>GSMELLQGKTFVVMGVANQRSIAWGIARSLHNAGAKLIFTYAGERLERNVRELADTLEGQESLVLPCDVTNDEELTACFETIKQEVGTIHGVAHCIAFANRDDLKGEFVDTSRDGFLLAQNISAFSLTAVAREAKKVMTEGGNILT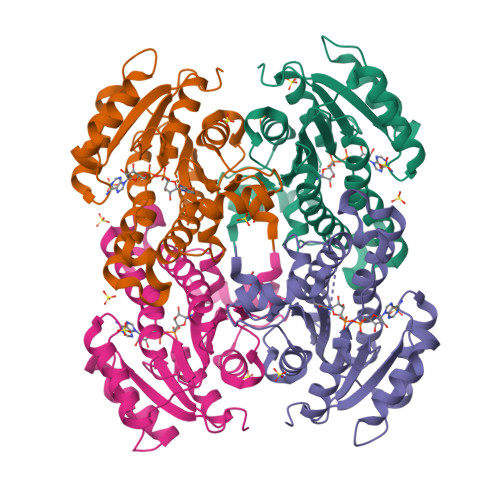LTYLGGERVVKNYNVMGVAKASLEASVKYLANDLGQHGIRVNAISAGPIRTLSAKGVGDFNSILREIEERAPLRRTTTQEEVGDTAVFLFSDLARGVTGENIHVDSGYHILG[4x]> MGSPASDPTVFHKRYLKKIRDLGEGHFGKVSLYCYDPTNDGTGEMVAVKALKADAGPQHRSGWKQEIDILRTLYHEHIIKYKGCCEDAGAASLQLVMEYVPLGSLRDYLPRHSIGLAQLLLFAQQICEGMAYLHAQHYIHRNLAARNVLLDNDRLVKIGDFGLAKAVPEGHEYYRVREDGDSPVFWYAPECLKEYKFYYASDVWSFGVTLYEL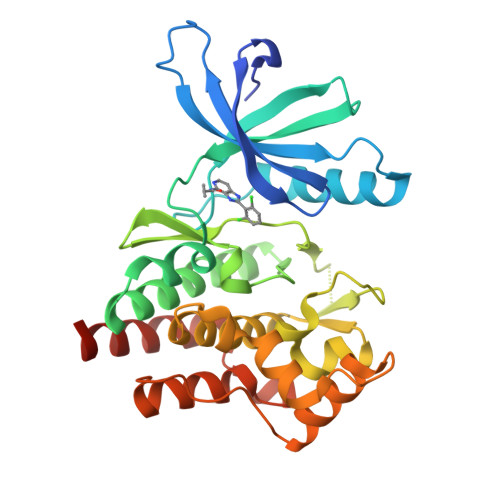LTHCDSSQSPPTKFLELIGIAQGQMTVLRLTELLERGERLPRPDKCPAEVYHLMKNCWETEASFRPTFENLIPILKTVHEKYRHHHHHH>[8x]GHMSTLLINQPQYAWLKELGLREENEGVYNGSWGGRGEVITTYCPANNEPIARVRQASVADYEETVKKAREAWKIWADIPAPKRGEIVRQIGDALREKIQVLGSLVSLEMGKILVEGVGEVQEYVDICDYAVGLSRMIGGPILPSERSGHALIEQWNPVGLVGIITAFNFPVAVYGWNNAIAMICGNVCLWKGAPTTSLISVAVTKIIAKVLEDNKLPGAICSLTCGGADIGTAMAKDERVNLLSFTGSTQVGKQVGLMVQERFGRSLLELGGNNAIIAFEDADLSLVVPSALFAAV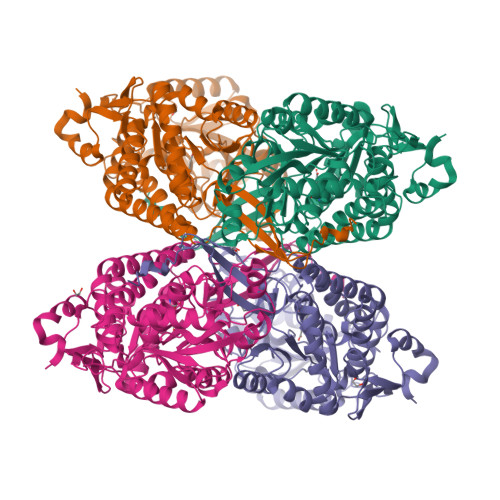GTAGQRCTTARRLFIHESIHDEVVNRLKKAYAQIRVGNPWDPNVLYGPLHTKQAVSMFLGAVEEAKKEGGTVVYGGKVMDRPGNYVEPTIVTGLGHDASIAHTDTFAPILYVFKFKNEEEVFAWNNEVKQGLSSSIFTKDLGRIFRWLGPKGSDCGIVNVNIPTSGAEIGGAFGGEKHTGGGRESGSDAWKQYMRRSTCTINYSKDLPLAQGIKFQ> GPGSGPVFVQEPSHVMFPLDSEEKKVKLSCEVKGNPKPHIRWKLNGTDVDIGMDFRYSVVDGSLLINNPNKTQDAGTYQCIATNSFGTIVSREAKLQFAYLENFKTRTRSTVSVRRGQGMVLLCGPPPHSGELSYAWIFNEYPSYQDNRRFVSQETGNLYIAKVEKSDVGNYTCVVTNTVTNHKVLGPPTPLILRNDGVMGEYEPKIEVQFPETVPAEKGTTVKLECFALGNPVPTILWRRADGKPIARKARRHKSNGILEIPNFQQEDAGSYECVAENSRGKNVAKGQLTFYAQPNWVQIINDIHVAMEESVFWECKANGRPKPTYRWLKNGDPLLTRDRIQIEQGTLNITIVNLSDAGMYQCVAENKHGVIFSSAELS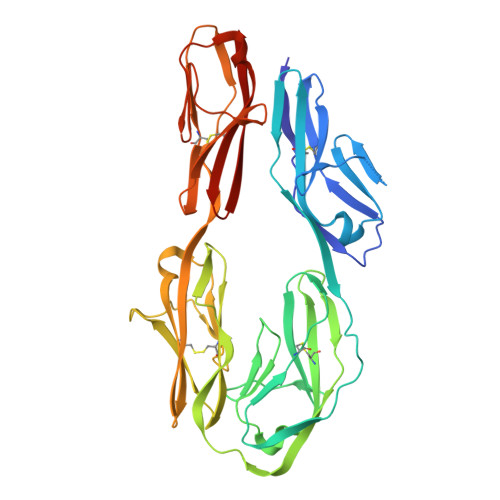VIAE>MEIISPIITPFDKQGKVNVDALKTHAKNLLEKGIDAIFVNGTTGLGPALSKDEKRQNLNA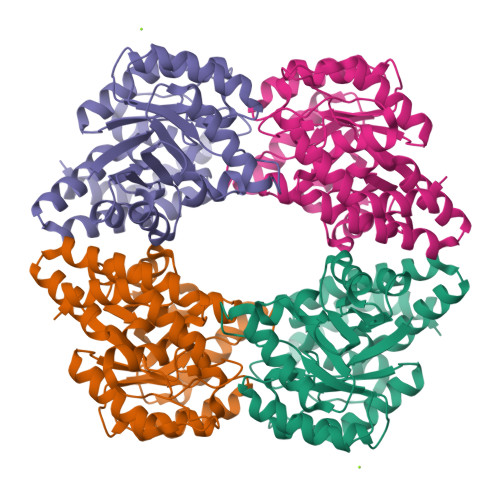LYDVTHKLIFQVGSLNLNDVMELVKFSNEMDILGVSSHSPYYFPRLPEKFLAKYYEEIARISSHSLYIYNYPAATGYDIPPSILKSLPVKGIKDTNQDLAHSLEYKLNLPGVKVYNGSNTLIYYSLLSLDGVVASFTNFIPEVIVKQRDLIKQGKLDDALRLQELINRLADILRKYGSISAIYVLVNEFQGYDVGYPRPPIFPLTDEEALSLKREIEPLKRKIQELVH[2x]>[3x]ASNFTQFVLVDNGGTGDVTVAPSNFANGVAEWISSNSRSQAYKVTCSVRQ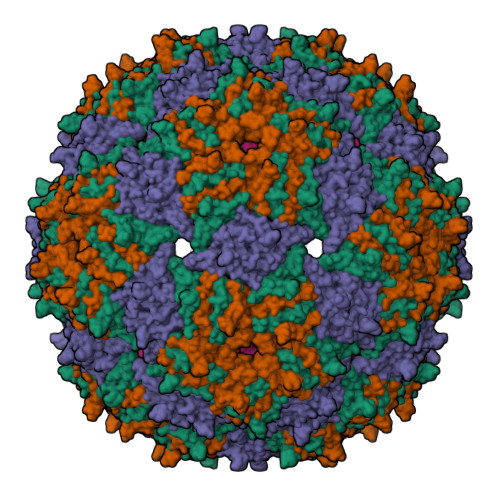SSAQNRKYTIKVEVPKVATQTVGGVELPVAAWRSYLAMKLTIPIFATNSDCELIVKAMQGLLKDGNPIPSAIAANSGIY>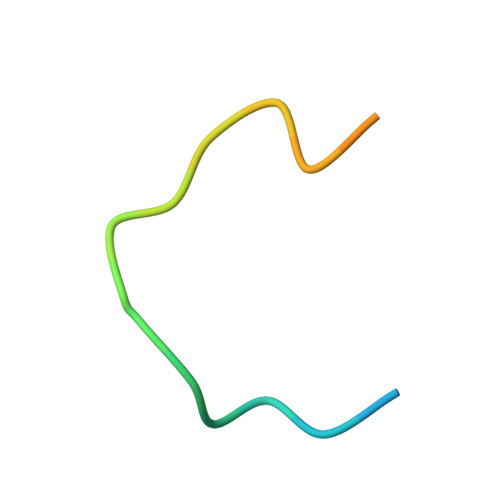 RDNATCDGPCGLRFRQKLESGMR> XLASFLMQAL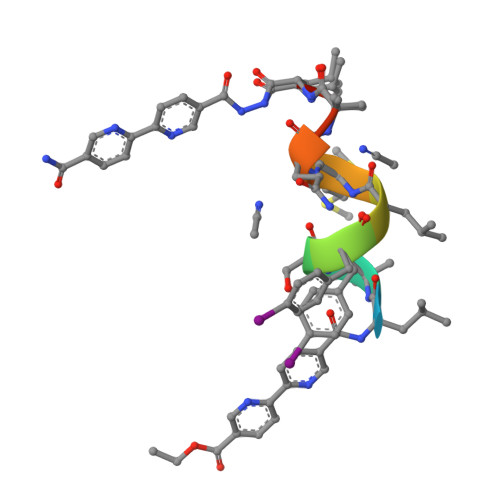X>[2x]MRLLHTMLRVGDLQRSID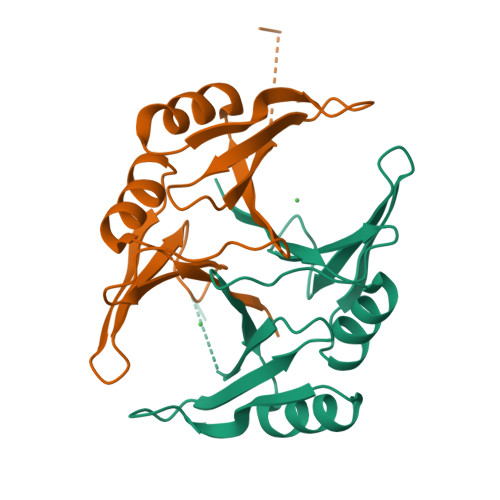FYTKVLGMKLLRTSENPEYKYSLAFVGYGPETEEAVIELTYNWGVDKYELGTAYGHIALSVDNAAEACEKIRQNGGNVTREAGPVKGGTTVIAFVEDPDGYKIELIEEKDAGRGLGN> GAMDPEFQQSKVAPSSAASRPVLSSRSDQSQKNEVFLDVVERLSVLIASNGSLLKVDVQGEIRLKSFLPSGSEMRIGLTEEFSVGKSELRGYGPGIRVDEVSFHSSVNLDEFESHRILRLQPPQGELTVMRYQLSDDLPSPLPFRLFPSVQWDRGSGRLQVYLKLRCDLLSKSQALNVRLHLPLPRGVVSLSQELSSPEQKAELAEGALRWDLPRVQGGSQLSGLFQMDVPGPPGPPSHGLSTSASPLGLGPASLSFELPRHTC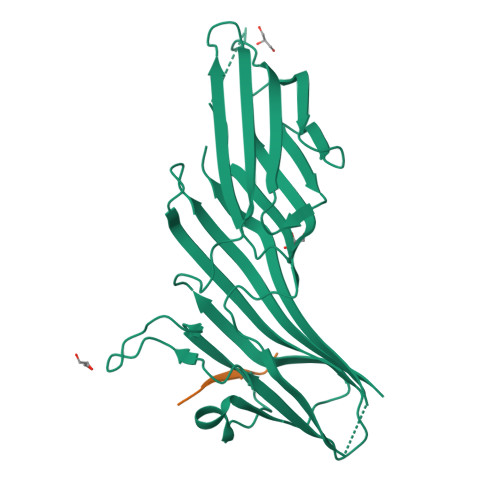SGLQVRFLRLAFRPSGNANPHKWVRHLSHSDAYVIRI;> TYKFFEQ> GTSTQTKAGSLTIVGTGIESIGQMTLQALSYIEAAAKVFYCVIDPATEAFILTKNKNCVDLYQYYDNGKSRLNTYTQMSELMVREVRKGLDVVGVFYGHPGVFVNPSHRALAIAKSEGYRARMLPGVSAEDCLFADLCIDPSNPGCLTYEASDFLIRDRPVSIHSHLVLFQVGCVGIADFNFTGFDNNKFGVLVDRLEQEYGAEHPVVHYIAAMMPHQDPVTDKYTVAQLREPEIAKRVGGVSTFYIPPKARKASNLDIIRRLELLPAGQVPDKKARIYPANQWEPDVPEVEPYRPSDQAAIAQLADHAPPEQYQPLATSKAMSDVMTKLALDPKALADYKADHRAFAQSVPDLTPQERAALELGDSWAIRCAMKNMPSSLLDAARESGEEASQNGFPWVIVVGPIGVIGS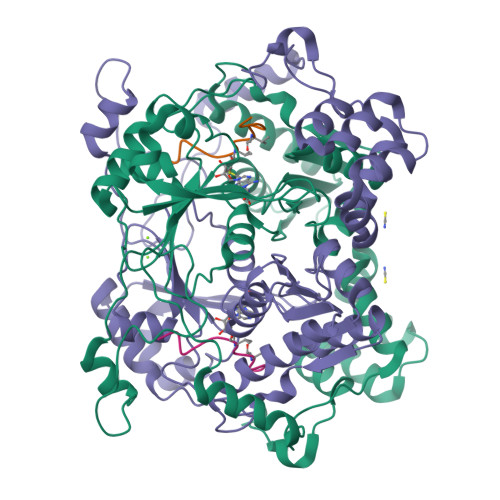VMSTE;> NGFPWVIVVGPIGVIGSVMSTE>[2x]GSTGSNASSQLTLLIGNLIQILGEKSLTALTNKITAWKSQQQARQQKNLEFSDK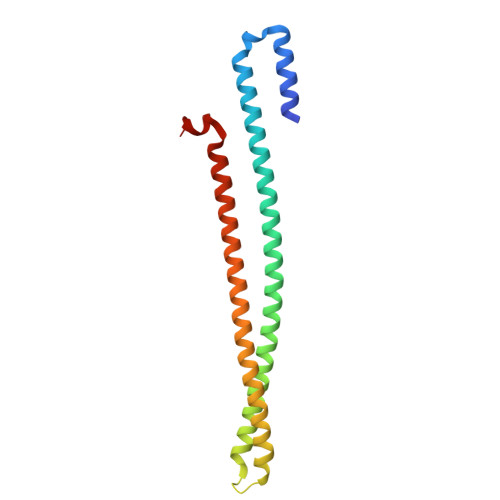INTLLSETEGLTRDYEKQINKLKNADSKIKDLENKINQIQTRLSELDPESPEKKKLSREEIQLTIKKDAAVKDRTLIEQKTLSIHSKLTDKSMQLEKEIDSFSAFSNTASAEQLSTQQKS2'-chloro-6-methyl[1,1'-biphenyl]-3-amine 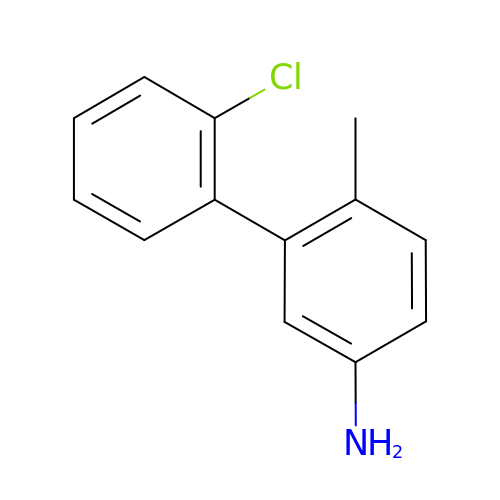| C13 H12 Cl N | QLKVQWRDOWGQQP-UHFFFAOYSA-N>[2x]METIQELILSEENKTNIAVLNLGTNDRRNAVLILETALHLVEKYLGKIINTSYLYETVPEYIVLDKKESCEKINKDCRIYDVNYINELMQNLEESKYEENKELIDKCEEYETFLKNGKVDNSILKEVNVENYLLECNNIIVKNDEIMKNNLSKYKDKYYTSYFYNLTVVVKTFVNDPLSMLV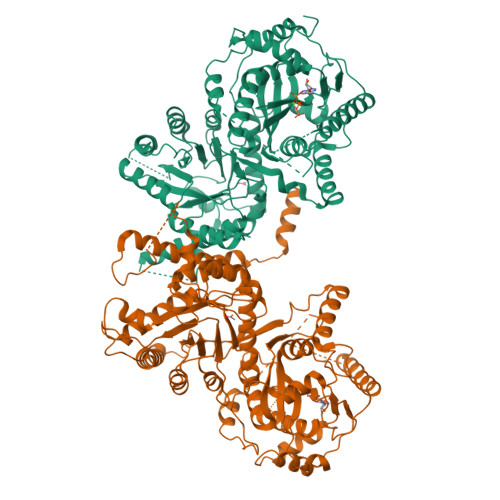VIKYIEELMKRENVKEKEKFENRIIDIDILFFNDFTIFMKNIKLEKNMIYKILSKYIHLERDIKNGNDNMSKVNMDKDINLNNNNNIKKKNNNDIDCDCVDQKMNNHVNNKNYINSFRDPQEIINNMVDNIEFLSIPHVYTTHRYSILLCLNDMIPEYKHNVLNNTIRCLYNKYVSRMKEQYNINIKENNKRIYVLKDRISYLKEKTNIVGILNVNYDSFSDGGIFVEPKRAVQRMFEMINEGASVIDIGGESSAPFVIPNPKISERDLVVPVLQLFQKEWNDIKNKIVKCDAKPIISIDTINYNVFKECVDNDLVDILNDISACTNNPEIIKLLKKKNKFYSVVLMHKRGNPHTMDKLTNYDNLVYDIKNYLEQRLNFLVLNGIPRYRILFDIGLGFAKKHDQSIKLLQNIHVYDEYPLFIGYSRKRFIAHCMNDQNVVINTQQKLHDEQQNENKNIVDKSHNWMFQMNYMRKDKDQLLYQKNICGGLAIASYSYYKKVDLIRVHDVLETKSVLDVLTKIDQVKDPNSSSVDKLAAALEHHHHHH>[2x]ETGFVNKDQIAKDVKQFYDQALQ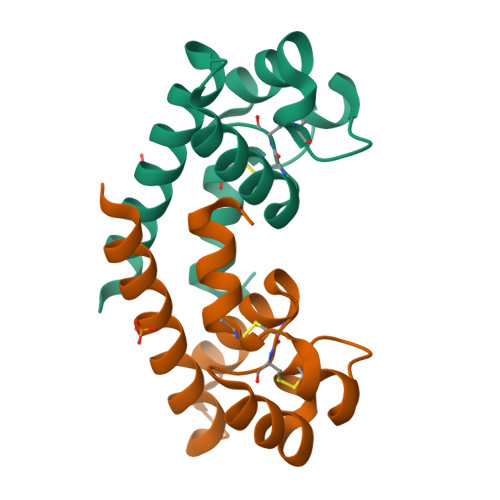QAVVDDDANNAKAVVKTFHETLDCCGSSTLTALTTSVLKNNLCPSGSNIISNLFKEDCHQKIDDLFSGKGTKHHHHHH>SSPCPQAWGPPGVQYGQPGRSVKLCCPGVTAGDPVSWFRDGEPKLLQGPDSGLGHELVLAQADSTDEGTYICQTLDGALGGTVTLQLGYPPARPVVSCQAADYENFSCTWSPSQISGLPTRYLTSYRKKTVLGADSQRRSPSTGPWPCPQDPLGAARCVVHGAEFWSQYRINVTEVNPLGASTRLLDVSLQSILRPDPPQGLRVESVPGYPRRLRASWTYPASWPSQPHFLLKFRLQYRPAQHPAWSTVEPAGLEEVITDAVAGLPHAVRVSARDFLDAGTWSTWSPEAWGTPSTGTIPKEIPAWGQLHTQPEVEPQVDSPA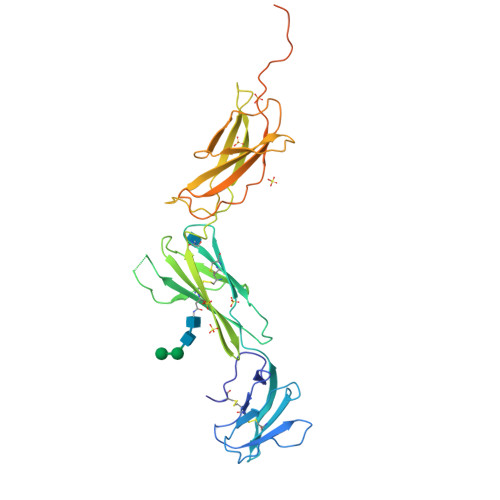PPRPSLQPHPRLLDHRDSVHHHHHHHH[2x]> AKLVFF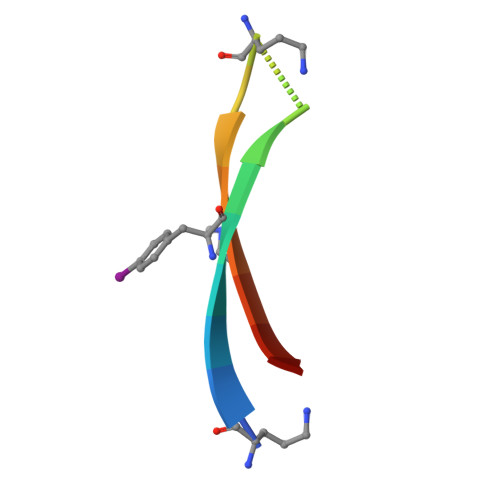AEAAIIGLMVV> GQSLRSFQKQNEDNDKRQQILRSINVNVSSSEAETKYNELIKEAFLVNENGEKVEGDAFATDVVKAATEHQYPVFVANVDGQPKYIMALHGAGLWGPLWGYISVDSDKNTIYGADFSHQGETPGLGAEISK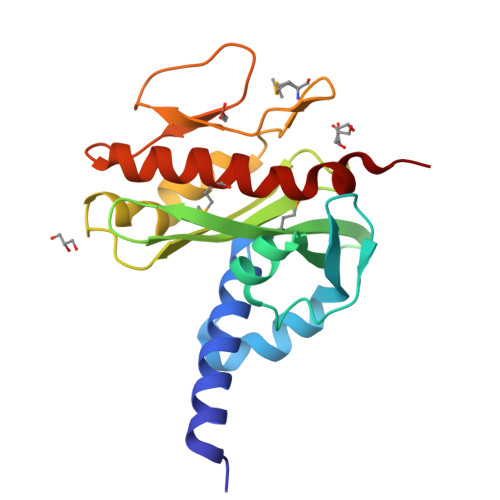PVFSNEFKGKKIFMSGEFKSVAVVKPGKSVAGQDYVDGISGGTITSKGVDEMLFNSLSGYVKFLTSQN N-[4-({3-[5-fluoro-2-(methylideneamino)pyrimidin-4-yl]pyridin-2-yl}oxy)phenyl]-2-(phenylamino)benzamide 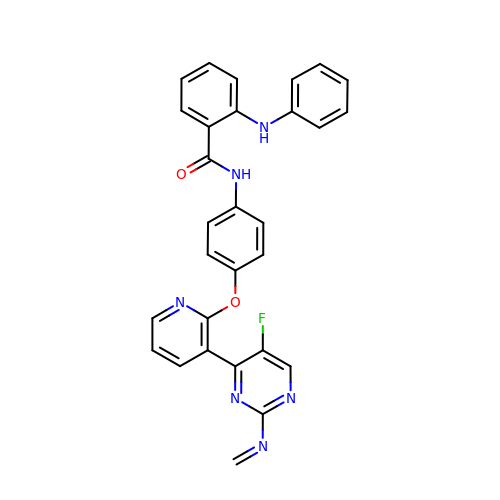| C29 H21 F N6 O2 | VGOJUQQDRYARLG-UHFFFAOYSA-N> MKKLLPILIGLSLTGFSAMSQAENLLQVYQQARISNPDLRKSAADRDAAFEKINEARSPLLPQLGLGADYTYTSGFRDYKDQNSNVTSGSLQLTQVLFDMSKWRALTLQEKAAGIQDVTYQTDQQTLILNTATAYFKVLAAIDTLSYTEAQKQAIYRQLDQTTQRFNVGLVAITDVQNARSQYDAVLANEVTARNDLDNAVEELRQVTGNYYPELASLNVDGFKTSKPQAVNALLKEAENRNLSLLQARLNQDLAREQIRQAQDGHLPTLDLNASSGVSNNRYSGSKSISQDADIGQNKIGLSFSLPLYQGGMVNSQVKQAQYNFVGASEQLESAHRSVVQTVRSSFNNVNASISSINAYKQAVVSAQSSLDAMEAGYSVGTRTIVDVLDATTTLYNAKQQLSNARYNYLINELNIKSALGTLN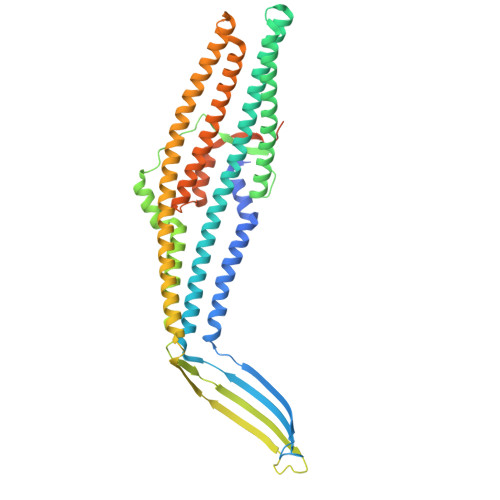EQDLIALNNTLGKPISTSADSVAPENPQQDATADGYGNTTAAMKPASARTTTHSSGSNPFRQLEHHHHHH The particles harbour 10-separate genome segments and comprise two principle protein layers, the innermost composed of 120 copies of protein λ1 clamped together by 150 copies of σ2 (viral polymerases, λ3, are attached inside adjacent to the icosahedral fivefold axes). The outer layer consists of 600 copies each of μ1 and σ3. The array of μ1 and σ3 is interrupted at the fivefold axes by pentameric λ2 turrets which enzymatically cap the mRNA transcripts produced by the polymerase on egress from the particle. Here we demonstrate that vitrification of infected cells followed by cryo-focussed ion beam (cryo-FIB) milling and cryo-electron tomography (cryo-ET) allows high resolution reconstruction of assembly intermediates of a mammalian reovirus, allowing atomic models to be constructed which throw light on some of these fundamental questions.

The star shaped icosahedral particles comprise 120 major proteins with additional density features on the outside. Since the 60 copies each of the A and B molecules account for the large majority of the density for these particles we henceforth term them single-layered particles (SLPs). The maximum diameter of the SLPs is very similar to the corresponding layer of virion-like particles, however whilst the latter are roughly spherical the SLP is collapsed inwards at the icosahedral fivefolds by 100 Å, to give the characteristic star shaped cross-section. Due to the radically different configurations of the SLP and virion-like particle the contacts between the molecules differ markedly between the two particles. Overall the contacts in the SLP are significantly weaker, with different residues involved. For the AB interface the rotation of the iris blades again radically alters the interface towards the fivefold axes, in this case through an unusual ratchet mechanism. If the A molecule is considered fixed then the change corresponds to a 45° rotation around a pivot helix in B, with the effect that a bundle of helices surrounding the pivot helix rotate by a register of one helix (~12 Å), analogous to gears slipping by one tooth. The 120 copies of λ1 are decorated with additional density at 120 sites. The density is poorly defined and only the region fairly close to the λ1 shell is seen, so it is not possible to unambiguously assign it to a particular protein however the overlap between the positions of these features and the attachment points of σ2 in the virus suggests that they are σ27. There are no significant sites of unexplained density in the interior of the λ1 layer of the SLP that might be attributed to the λ3 polymerase.

>QRHITEFISSWQNHPIVQVSADVENKKTAQLLHADTPRLVTWDAGLCTSFKIVPIVPAQVPQDVLAYTFFTSSYAIQSPFPEAAVSRIVVHTRWASNVDFDRDSSVIMAPPTENNIHLFKQLLNTETLSVRGANPLMFRANVLHMLLEFVLDNLYLNRHTGFSQDHTPFTEGANLRSLPGPDAEKWYSIMYPTRMGTPNVSKICNFVASCVRNRVGRFDRAQMMNGAMSEWVDVFETSDALTVSIRGRWMARLARMNINPTEIEWALTECAQGYVTVTSPYAPSVNRLMPYRISNAERQISQIIRIMNIGNNATVIQPVLQDISVLLQRISPLQIDPTIISNTMSTVSESTTQTLSPASSILGKLRPSNSDFSSFRVALAGWLYNGVVTTVIDDSSYPKDGGSVTSLENLWDFFILALALPLTTDPCAPVKAFMTLANMMVGFETIPMDNQIYTQSRRASAFSTPHTWPRCFMNIQLISPIDAPILRQWAEIIHRYWPNPSQIRYGAPNVFGSANLFTPPEVLLLPIDHQPANVTTPTLDFTNELTNWRARVCELMKNLVDNQRYQPGWTQSLVSSMRGTLDKLKLIKSMTPMYLQQLAPVELAVIAPMLPFPPFQVPYVRLDRDRVPTMVGVTRQSRDTITQPALSLSTTNTTVGVPLALDARAITVALLSGKYPPDLVTNVWYADAIYPMYADTEVFSNLQRDMITCEAVQTLVTLVAQISETQYPVDRYLDWIPSLRASAATAATFAEWVNTSMKTAFDLSDMLLEPLLSGDPRMTQLAIQYQQYNGRTFNVIPEMPGSVIADCVQLTAEVFNHEYNLFGIARGDIIIGRVQSTHLWSPLAPPPDLVFDRDTPGVHIFGRDCRISFGMNGAAPMIRDETGMMVPFEGNWIFPLALWQMNTRYFNQQFDAWIKTGELRIRIEMGAYPYMLHYYDPRQYANAWNLTSAWLEEITPTSIPSVPFMVPISSDHDISSAPAVQYIISTEYNDRSLFCTNSSSPQTIAGPDKHIPVERYNILTNPDAPPTQIQLPEVVDLYNVVTRYAYETPPITAVVMGVP[2x]>[4x]MNINEILKKLINKSDLEINEAEELAKAIIRGEVPEILVSAILVALRMKGESKNEIVGFARAMRELAIKIDVPNAIDTAGTGGDGLGTVNVSTASAILLSLVNPVAKHGNRAVSGKSGSADVLEALGYNIIVPPERAKELVNKTNFVFLFAQYYHPAMKNVANVRKTLGIRTIFNILGPLTNPANAKYQLMGVFSKDHL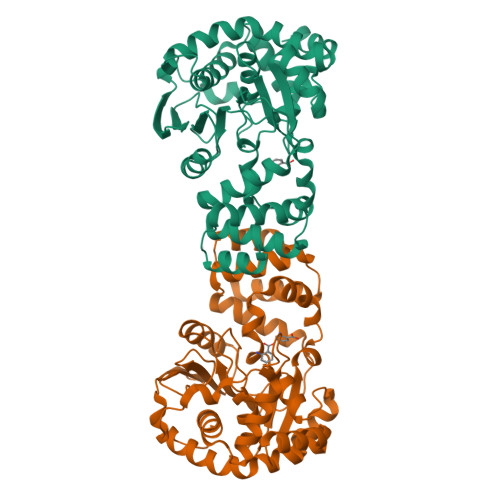DLLSKSAYELDFNKIILVYGEPGIDEVSPIGNTFMKIVSKRGIEEVKLNVTDFGISPIPIEKLIVNSAEDSAIKIVRAFLGKDEHVAEFIKINTAVALFALDRVGDFREGYEYADHLIEKSLDKLNEIISMNGDVTKLKTIVVKSSG> MTISTPVIIDSLIRHAQRTPEQTALLCGDQHWNYRQLVTRAHVMASALRQAGLSGQAILLNLPKSLDAVAAIYATWLSGNHYIPIDYSQPSSRIERIIAAAAPALIIDTAWLATLDSQPSFDAEQPVGRMVYHNPIAAILYTSGSTGTPKGVQISHEMLGFFIQWAVRDTQLTARDVLSNHASFAFDLSTFDLFASAYVGAATWIIRESEQKDCAALAQGLQRHAVSVWYSVPSILAMLEKSTLLNPTLGQSLRQVIFAGEPYPVTALKRLLPCLPQPCRVSNWYGPTETNVCVAYAIDRARLAMLKQVPIGLPLEGLTAQLEDENGDRHPLTAQLRLSGELLISGPCVTPG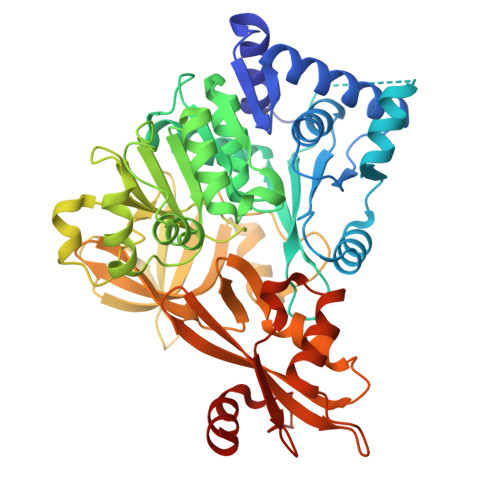YSNVVVPRQAALHPHQCHATGDWVEMTPEGLVFRGRIDDMVKINGYRVELGEIESVLHQHPAIDRAALCVELGDLRQTLIMVISLQTGAVPPGLLELKQFLQQKLPSYMIPNKLVITESLPVNANGKVDRKQLAGVVAVLEHHHHHH> MKLTPKELDKLMLHYAGELAKKRKEKGIKLNYV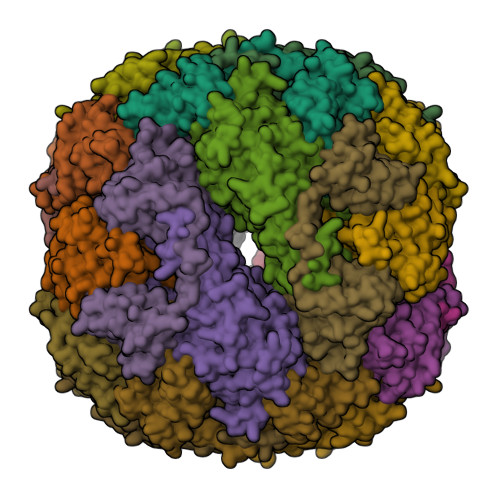EAVALISAHIMEEARAGKKTAAELMQEGRTLLKPDDVMDGVASMIHEVGIEAMFPDGTKLVTVHTPIEANGKLVPGELFLKNEDITINEGKKAVSVKVKNVGDRPVQIGSHFHFFEVNRCLDFDREKTFGKRLDIAAGTAVRFEPGEEKSVELIDIGGNRRIFGFNALVDRQADNESKKIALHRAKERGFHGAKSDDNYVKTIKE;> MKKISRKEYVSMYGPTTGDKVRLGDTDLIAEVEHDYTIYGEELKFGGGKTLREGMSQSNNPSKEELDLIITNALIVDYTGIYKADIGIKDGKIAGIGKGGNKDMQDGVKNNLSVGPATEALAGEGLIVTAGGIDTHIHFISPQQIPTAFASGVTTMIGGGTGPADGTNATTITPGRRNLKWMLRAAEEYSMNLGFLAKGNASNDASLADQIEAGAIGFKIHEDWGTTPSAINHALDVADKYDVQVAIHTDTLNEAGCVEDTMAAIAGRTMHTFHTEGAGGGHAPDIIKVAGEHNILPASTNPTIPFTVNTEAEHMDMLMVCHHKDKSIKEDVQFADSRIRPQTIAAEDTLHDMGAFSITSSDSQAMGRVGEVITRTWQTADKNKKEFGRLKEEKGDNDNFRIKRYLSKYTINPAIAHGISEYVGSVEVGKVADLVLWSPAFFGVKPNMIIKGGFIALSQMGDANASIPTPQPVYYREMFAHHGKAKYDANITFVSQAAYDKGIKEELGLERQVLPVKNCRNVTKKDMQFNNTTAHIEVNPETYHVFVDGKEVTSKPANKVSLAQLFSIF2,4,6-TRIAMINOQUINAZOLINE | C8 H9 N5 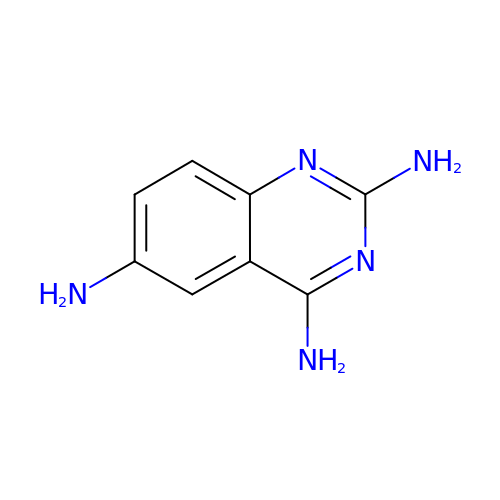| LJBWEZVYRBKOCI-UHFFFAOYSA-N Proteomic analysis of ES products of adult H. polygyrus revealed that the most abundant proteins are members of the venom allergen-like protein (VAL) family, and among the major ones is H. polygyrus VAL-4 (HpVAL-4). VALs are members of the superfamily that is known as CAP (cysteine-rich secretory protein/antigen 5/pathogenesis related-1) or SCP/TAPS (Sperm-coating protein/Tpx/antigen 5/pathogenesis related-1/Sc7). There are >30 secreted Heligmosomoides polygyrus VAL proteins (HpVALs) and these proteins are characterised by having either one or two 15 kDa CAP (cysteine-rich secretory protein (CRISP)/antigen 5/pathogenesis related-1) domains. HpVAL-4 has both palmitate-binding and sterol-binding cavities and is able to complement the in vivo sterol export phenotype of yeast mutants lacking their endogenous CAP proteins.

The first known HpVAL structure, HpVAL-4, refined to 1.9 Å is reported. HpVAL-4 was produced as a homogeneously glycosylated protein in leaves of Nicotiana benthamiana infiltrated with recombinant plasmids, making this plant expression platform amenable for the production of biological products. The overall topology of HpVAL-4 is a three layered αβα sandwich between a short N-terminal loop and a C-terminal cysteine rich extension. While the refined model has four monomers of HpVAL-4 in the asymmetric unit, this tetramer is likely an artefact of crystallisation as SEC-MALS analysis indicates that HpVAL-4 is a monomer in solution. The predicted N-linked glycosylation site Asn12 is glycosylated for all four monomers. The surface plot of HpVAL-4 reveals a large central CAP cavity of 1732.64 Å3, which is bordered by the first beta strand (β1) and the third and fourth alpha helices (α2,α4), and opens into a C-terminal loop. HpVAL-4 shares a conserved C-terminal extension with Na-ASP-2 that has two strands, which are stabilised by two disulfide bonds. The flexible N-terminal loops of both proteins also have a conserved disulfide bond with alpha helix 2. HpVAL-4 has a large central cavity that lacks the prototypical CAP cavity tetrad, which means it will be incapable of binding divalent cations. The amino acid residues in the CAP cavity of HpVAL-4 are more similar to those in the amino terminal CAP domain of the two CAP Na-ASP-1.

>[4x]SEFGCDGTLEQNDTTREVFLRFHNDVRKFIALGIYPNKVGVLGPAKNMYQLKWSCDLEEEAHESIYSCSYNPLLLHPQSYSKLLSVDLPDTDVVGATLEMWTEFMRIYGVNTKTNSYNPSFSQFANMAYSKNTKVGCSYKKCGGDTLVTCVYELGVKLPSHPQMWENGPTCVCVAYTDSICNDNNLCEYAPTSAR> MADDFAY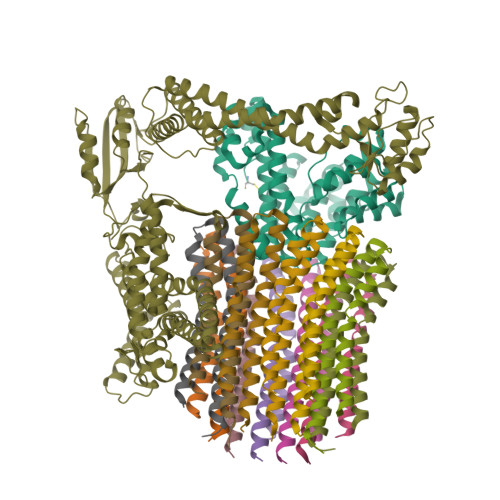LNARVRVRRGTLLKESFFQEALDLSFADFLRLLSETVYGGELAGQGLPDVDRAVLRTQAKLVGDLPRLVTGEAREAVRLLLLRNDLHNLQALLRAKATGRPFEEVLLLPGTLREEVWRQAYEAQDPAGMAQVLAVPGHPLARALRAVLRETQDLARVEALLAKRFFEDVAKAAKGLDQPALRDYLALEVDAENLRTAFKLQGSGLAPDAFFLKGGRFVDRVRFARLMEGDYAVLDELSGTPFSGLSGVRDLKALERGLRCVLLKEAKKGVQDPLGVGLVLAYVKEREWEAVRLRLLARRAYFGLPRAQVEEEVVCP;> MIAPMEKLVLAGPKGRAKELLQSLQQAGVVHLETLRPEALSAYQLSPEERAELRRWEAVSAGAEHTLSLLGLEAEPARPFPEGLEAAEKALSPIQAHAEGLTRQKQELEEELALAQAYLEPLERLAALAHGLDKSPFLRVIPFLLTEKELPLVEEALRKALEDRYLLAHEAYAGGVAALVVVHRKEVDQAKAALSRAGVAELRLPGALGELPLSEAARRLKERAEAAPRELSEVRQHLAKLARESASTLQSLWTRAQDEVARLKALEELASGRFGFALLGYVPVKAKPKVEEALARHKESVVYAFEPVDEHHEADRIPVVLDNPPWAKPFELLVSFLNTPKYGTFDPTPVVPVFFPFWFGMIVGDIGYALLFYLVGRWLSGYVKRNEPLVIDLFALKLKPQVIGKLVHILNWMVFWTVVWGVIYGEFFGTFLEHLGVFGTPEHPGLIPILIHRIDTAKTANLLILLSVAFGVVLVFFGLALRAYLGLKHRHMAHFWEGVGYLGGLVGVLALAASYLGNLQAGWLQGLMYLGFGVFLLAVLMSRIWLMIPEIFTQAGHILSHIRIYAVGAAGGILAGLLTDVGFALAERLGLLGVLLGLLVAGVLHLLILLLTTLGHMLQPIRLLWVEFFTKFGFYEENGRPYRPFKSVREAQ;>[12x]MKKLLVTVLLAVFGALAFAAEEAAASGGLDRGLIAVGMGLAVGLAALGTGVAQARIGAAGVGAIAEDRSNFGTALIFLLLPETLVIFGLLIAFILNGRLHHH>[2x]MELWLVRHGETLWNREGRLLGWTDLPLTAEGEAQARRLKGALPSLPAFSSDMLRARRTAELAGFSPRLYPELREIHFG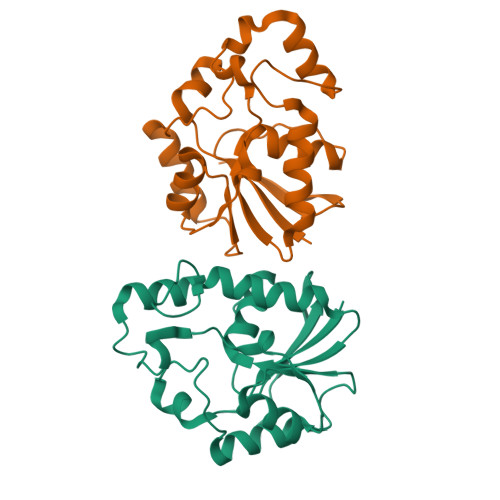ALEGALWETLDPRYKEALLRFQGFHPPGGESLSAFQERVFRFLEGLKAPAVLFTHGGVVRAVLRALGEDGLVPPGSAVAVDWPRRVLVRLALDGEEATG>SNAFLDYGLSEADPDVHAIINKEKDRQFRSLELIASENFTSKAVMEAVGSCLTNKYSEGLPGKRYYGGNEHIDELEILCQQRALAAFHLDGDKWGVNVQPLSGSPANFAVYTAILKPHDRIMGLDLPHGGHLSHGFMTAKRRVSGTSIYFESMPYRLDESTGVIDYDMLEKTAALFRPKLIIAGASAYPRDIDYARFRKIADSVGAFLMMDMAHVSGLIAASVLADPFEFVDIVTTTTHKSLRGPRGGMIFFKKDAVHGVDLESAINNAVFPGLQGGPHNHTIGGLAVCLKYAQSPDFKNYQNQVVANCRALANRLVEHEYKLVSGGSDNHLVLVDLRPSGIDGARVEKILDMASITLNKNSVPGDKSALVPGGIRIG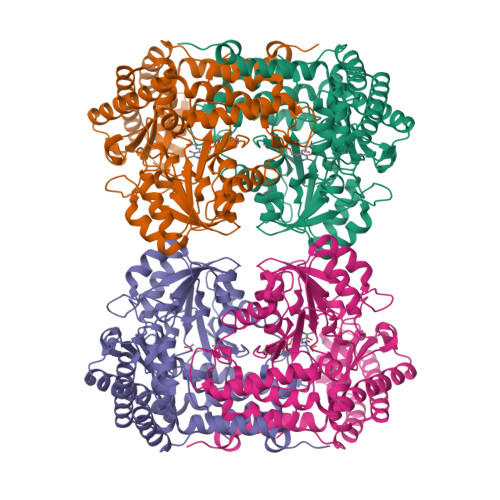SPAMTTRGLGEKEFELIADLIHEGVRISLEAKSLVSGTKVQDFLNFVLAPEFPLGDKVSNLRRKVEALATQYPIPGV[8x]> TTVTIVRKDGRIAIAADTLTKWGGGKESADYVANHEKIIRVGDSYVAITGSATFKLILADYFASLDEPPQLDSVARIFCVWNTLHGALKEHYYLQAGEDKEDDLESSRMDVLIANPRGIFGVAAHRTVQEFSKFYAYGSGSPYALGAMYAAYRAPSLDAEAVARLGVMAAAEFHDESGLPVQSFVMELSPDVG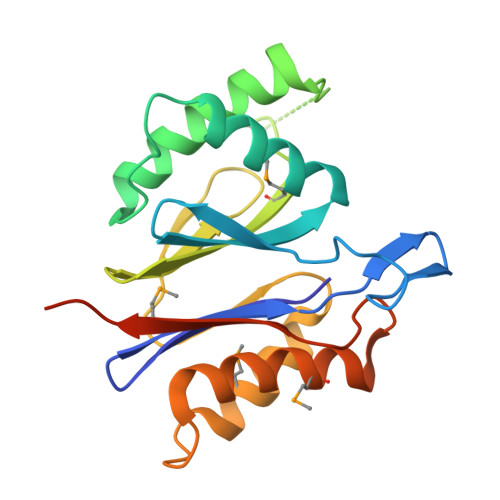SGENLYFQ URIDINE | 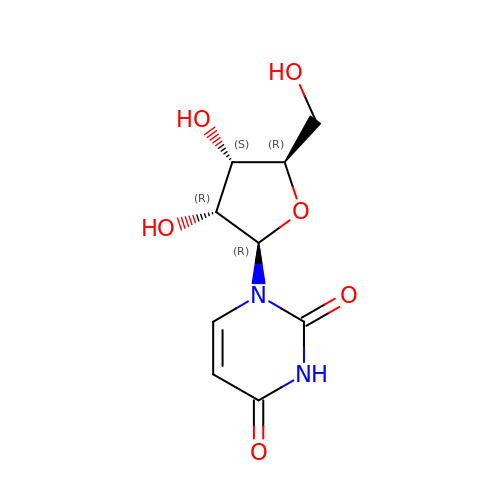C9 H12 N2 O6 | DRTQHJPVMGBUCF-XVFCMESISA-N> L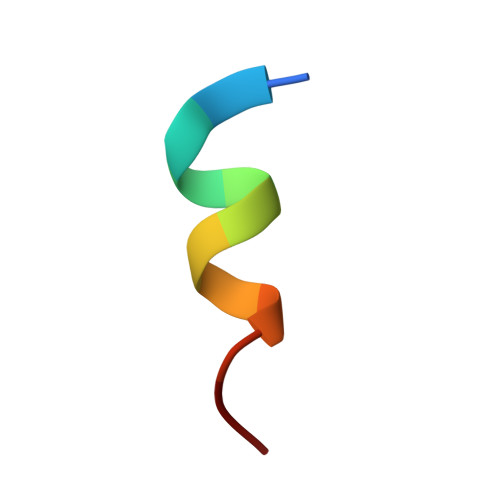TFEHYWAQLTS>MTDEKKVPSKPARPARKPRADKPADAKPAAVPKVAAPAVVEGSSTNAAAVKKSLRDGGMTALPSEILFAVGSIPLVVDKDALSTLAAALVASDDPSTWFVANRELIRAVVFVPQQNNVLRATPLLSVRPVASLSSVHNWQVRNHLSGLHVVVGGTGAGKSKWLNAQTPDVTIRWGEPGETFDMEESSIAVADLTEMLAVALLLATADYRVVIDSFRNLVFGITGAAGPGGVSVALYAALTSLNNICAELGVLLVAAINPMSSDDKVSLVYNNIAASVAGMTVVNNAAVVSQTIRSGTGRIFSGEPAPRNDSPVEYHEPRHTQLDEPSGPSARIRLESNNIDPDDENDNRPRRGARISL[6x]

The lipid-enveloped bacteriophages of the Cystoviridae family infect Gram-negative bacteria, mainly plant-pathogenic Pseudomonas species and share similarities with the members of the Reoviridae family, including bluetongue virus and rotavirus. Their genome of ∼14 kb consists of three dsRNA segments small (S), medium (M) and large (L), which are sequentially encapsidated as ssRNA precursors into the icosahedrally symmetric procapsid by the packaging NTPase P4 (15–23). P4 is a protein of ∼35 kDa, which can assemble into a hexameric ring. NTP-binding sites are located on the external perimeter of the ring at the interfaces between adjacent subunits, whereas the nucleic acid binding sites are found in the central channel. P4 proteins are the only known RNA-specific helicases belonging to helicase Superfamily 4 (SF4).

The ɸ6 P4 was crystallised with ADP-Mg2+ bound in the nucleotide binding site, whereas P4 from ɸ8 and ɸ13 were crystallized in their apo form. Most of the N-terminal domain residues of P4 from ɸ6 and ɸ8 are visible in our crystal structures (starting from amino acid residues 2 and 12, respectively), whereas ɸ13 P4 lacks the first 32 residues [which are predicted to be disordered (60)]. Interestingly, ɸ8 and ɸ13 P4s also lack such a stabilizing helix; however, the first 12 and 31 residues, respectively, are not visible in the crystal structures and might play such a stabilizing role. However in ɸ6 and ɸ13, more than half of their residues can be superimposed with a root-mean-square deviation of 2.1 Å, including two parallel helices and two small anti-parallel β-sheets, creating a topologically identical sub-domain. In ɸ6 and ɸ13, the C-termini are predicted to be disordered with little secondary structure, and indeed, no density for these domains could be found in our crystal structures. The structures of P4 from ɸ6 and ɸ13 show ordered L1 loops, which line the central channel and contact the L2 loops. The L2 loops are found with lysine residues (K239 and K265, respectively) projecting towards the centre of the channel, in the same position as K241 in ɸ12, suggesting a conserved mechanism for binding and translocating RNA. In P4 from ɸ6, ɸ12 and ɸ13, the arginine fingers are pointing towards the catalytic sites, making the subunits competent and primed for hydrolysis. From our structures, we predict similar loose arrangements in P4 from ɸ8 and ɸ13 where F247 (from the same subunit) and F301 (from a neighbouring subunit) seem to be in the correct orientation to stack the nucleotide base.>MARKTNIEAYRDGLKLKTEEDFFACDRQYVCQNYAPVPVVISKGKGARVWDINGNEYYDFLAGVSSLSQGHCHPRVIAALCRQAERLTLTLRAFGNDVTGPACRFMAEMFGYDRVLLMNTGAEAGESALKIARKWAYEVKEIPPDSAKVILCNNNYWGRTITACSSSTTFDCYNNFGPFTPGFELIDYDDVGALEEALKDPNVAAFFVEPIQGEGGVNVPKPGYLKRAHELCRSKNVLLIVDEIQTGLCRTGRLLAADHDEVHPDILLLGKSLSAGVVPISAVMGRADVMDVLKPGTHGSTFGGNPLACAVAVEALTVLKDEKLADRAERLGAQFRDCLRRELYGKVPWIKEIRGRGLLNAVEVDSDAIDPNDVVMKLKENGILSKPTRGRVMRFIPPLVITDEEHRDATTRIIKSFLAVEEERKKGENLYFQSAGHHHHHH[2x]

Toxoplasma gondii is one of the most significant parasites that impacts human health, with estimates that as many as one third to one half of the human population are infected. At the Center for Structural Genomics of Infectious Diseases (CSGID), the first Toxoplasma Structural Genomics Pipeline was established. The enzymes selected from the TDR database as small and tractable for expression and crystallization included: phosphoglycerate mutase II (hereafter referred to as PGM), nucleotide diphosphate kinase (NDK), ribulose phosphate 3-epimerase (RPE), ribose-5-phosphate isomerase (RPI), and ornithine aminotransferase (OAT). The genes encoding these enzymes were cloned, proteins expressed and purified, crystallized, and crystal structures were determined.

Ornithine aminotransferase, the final enzyme considered herein, is an enzyme involved in the urea cycle, TCA cycle, polyamine synthesis, and other pathways. It catalyzes a reversible reaction allowing interconversion of intermediates from ornithine to amino acids. Each monomer has a mixed α/β structural fold and consists of the cofactor PLP-binding domain (residues 87–336), an N-terminal domain (residues 17–86), and a C-terminal domain (residues 337–441). The dimerization interface is primarily formed between residues of the PLP-binding and N-terminal domains of TgOAT. The dimer is held by 3 salt bridges, Cys96–Cys96 disulfide bond, 63 hydrogen bonds and 782 van der Waals interactions. The cofactor-binding domain of TgOAT non-covalently binds PLP molecule, i.e., PLP does not form the Schiff base with conserve Lys286. Similarly to homologous OAT structures obtained in complex with the cofactor, PLP interacts with Thr135, Gly136, Ala137, Tyr171, Trp172, Glu224, Asp257, Ile259, Gln260, Lys286, Ser315, and Thr316. Most of these residues are highly conserved among TgOAT homologs and represent a viable, “druggable” pocket (SiteMap score 1.03). One 1,3,5-Tris(4-carboxyphenyl)benzene (BTB), polyethylene glycol (PEG) and acetate (ACT) molecule were modeled to interpret additional electron density in chain B. TgOAT appeared dispensable (fitness score of +1.2) in the tachyzoite CRISPR/Cas9 assays consistent with TgOAT appeared to be expressed predominantly in the oocyst stage (ToxoDB).> MNPAAEAEFNILLATDSYKVTHYKQYPPNTSKVYSYFECREKKTENSKLRKVKYEETVFYGLQYILNKYLKGKVVTKEKIQEAKDVYKEHFQDDVFNEKGWNYILEKYDGHLPIEIKAVPEGFVIPRGNVLFTVENTDPECYWLTNWIETILVQSWYPITVATNFREQKKILAKYLLETSGNLDGLEYKLHDFGYRGVSSQETAGIGASAHLVNFKGTDTVAGLALIKKYYGTKDPVPGYSVPAAEHSTITAWGKDHEKDAFEHIVTQFSSVPVSVVSDSYDIYNACEKIWGEDLRHLIVSRSTQAPLIIRPDS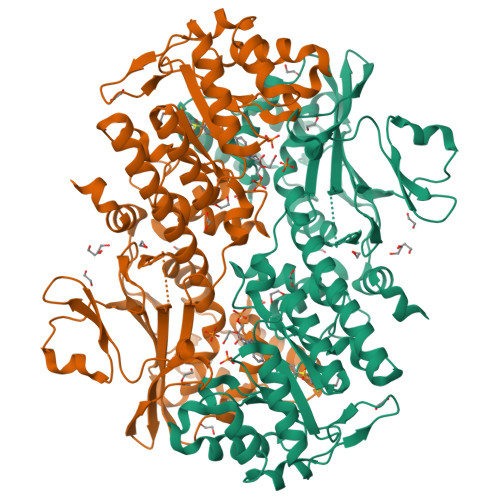GNPLDTVLKVLEILGKKFPVTENSKGYKLLPPYLRVIQGDGVDINTLQEIVEGMKQKMWSIENIAFGSGGGLLQKLTRDLLNCSFKCSYVVTNGLGINVFKDPVADPNKRSKKGRLSLHRTPAGNFVTLEEGKGDLEEYGQDLLHTVFKNGKVTKSYSFDEIRKNAQLNIELEAAHHLEHHHHHHHH>SMNENYLQAVKDSAKSQYASLRESYKSITGKTESADELPDHDAEVLDSIMDRLHEPLYEKDTFDPNEVLAENKQLYEEFLLQEISEPKVDNLVRSGDPLAGKAKGTILSLVRNSDLEDIISSIQQLEEEYNKNFGYPYTFLNDEEFTDEFKDGIKSILPKDRVVEFGTIGPDNWNMPDSIDRERYDQEMDKMSKENIQYAEVESYHNMCRFYSKEFYHHPLLSKYKYVWRLEPNVNFYCKINYDVFQFMNKNDKIYGFVLNLYDSPQTIETLWTSTMDFVEEHPNYLNVNGAFAWLKDNSQNPKNYDYTQGYSTCHFWTNFEIVDLDFLRSEPYEKYMQYLEEKGGFYYE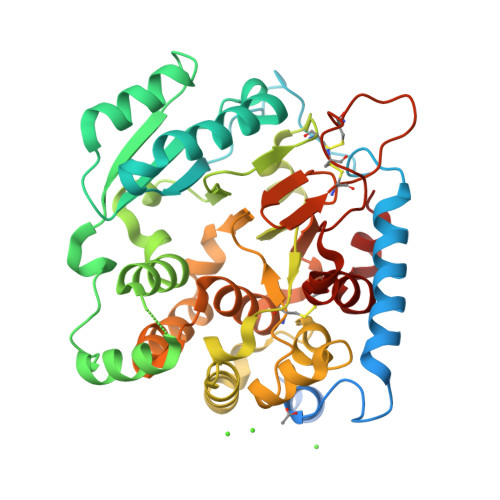RWGDAPVRSLALALFADKSSIHWFRDIGYHHTPYTNCPTCPADSDRCNGNCVPGKFTPWSDLDNQNCQATWIRHSMSEEELEMY[2x]> ME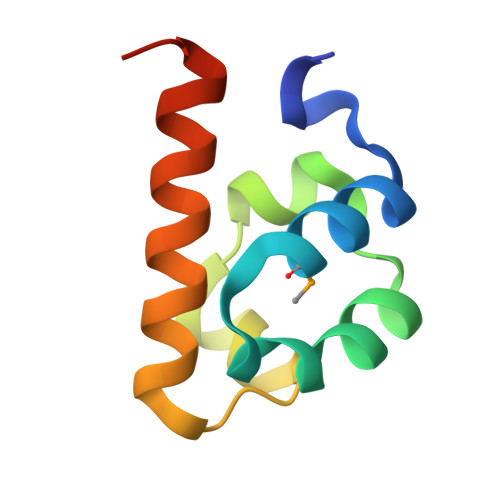PVSKWSPSQVVDWMKGLDDCLQQYIKNFEREKISGDQLLRITHQELEDLGVSRIGHQELILEAVDLLCALNYGLETEN>MANTGEMKINWVSRYMPLLNKIAEEYSREKPLSGFTVGMSIHLEAKTAYLAITLSKLGAKVVITGSNPLSTQDDVAEALRSKGITVYARRTHDESIYRENLMKVLDERPDFIIDDGGDLTVISHTEREEVLENLKGVSEETTTGVRRLKALEETGKLRVPVIAVNDSKMKYLFDNRYGTGQSTWDAIMRNTNLLVAGKNVVVAGYGWCGRGIALRAAGLGARVIVTEVDPVKAVEAIMDGFTVMPMKEAVKIADFVITASGNTDVLSKEDILSLKDGAVLANAGHFNVEIPVRVLEEIAVEKFEARPNVTGYTLENGKTVFLLAEGRLVNLAAG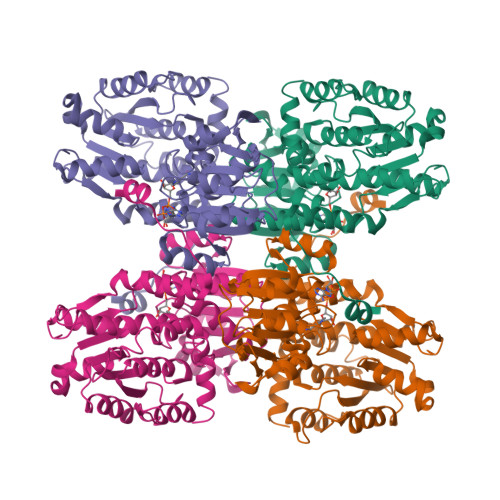DGHPVEIMDLSFALQIFAVLYLLENHRKMSPKVYMLPDEIDERVARMKLDSLGVKIDELTEKQRRYLRSWQHHHHHH[4x]>MKASLTFSLSGIYAPCSISRDIYLEYGDKKAECLYGTIRLPQYGPGCTPGKIVHCVLDDSLPFCSIVVPSKLFGFMPTQPTMDFCYFEPILDNVVPVLDSVTFLINEQLYSKLMDLPQEMQQIQFLHYKYNINSMETVVHSRDILTSGLCQILNCSPFPQGLVDFTETQLILVNDTEQKLSALKYANEDEEYALPKIGTNSALSIDLESLPCTISRDLLRPAPHINDDNSIYAFTDAETLLRLDVTSGSFITVSNMGCVRLVKLFVLLLPNGFKKRTIYAPPKIIASFPDCSVVTISKSNIGHTDIPIANQVFISRVGGWLQSQKCFQNIILTTLKKFFSESKRILCQNDLIPIAFDSSMADLNIAEENDESDDEDELGQYYKNDSLVWFFVTSAELDCFSKDNSHFIIDPNRTKLITTNITNRRPLPLSRSNLQRYYGFAETFYYDLHIFPYVRQLVNILETSFNCSQRGITLNASVLLHSTTNNVGKATMVRFASKYLGIHLLEIDCLSLTSNSRQLDSTSKIIGYIRAKCENVLPYASPAVIFLAHLDSILLDVNANQDPEAIKLQKSINFEMSKLLDDFTFKFPGTTFVGSVNNIDNVPSSFRSHMRFEILVPVPSEAQRLRIFQWYLSSHELNRDVQQKVPVSYMDNISFSSLSSYSAGLTPLDIKSIVETARMTATARFYQESKKCGWLPQSILITQEDLSKATSKARNEFSVSIGAPQIPNVTWDDIGGIDFVKGEILDTIDMPLKHPELFTSGMKKRSGILFYGPPGTGKTLMAKAIATNFSLNFFSVKGPELLNMYIGESEANVRRVFQKAREAKPCVIFFDQIDSVAPKRGNQGDSGGVMDRIVSQLLAELDGMSTDADGVFVIGATNRPDLLDEALLRPGRFDKLLYLGIPDTDTKQLNILEALTRKFVLDNDVKLIELAKLCPFNYTGADFYALCSDAMLNAMSRIARMVEKKVSQHNELTGENISTRRWFDKIATKEDTKVVVKMEDFLKAQEQLTPSVSRAELNHYEAVRANFEGA[3x];>TILKNGAIQLLKKVILRSTVCKMDFPKDNLFVVYISDGAQLPSQKGYASIVKCSLRQSKKSDSDNKSVGIPSKKIGVFIKCDSQIPENHIALSSHLWDAFFTHPMNGAKIKLEFLQMNQANIISGRNATVNIKYFGKDVPTKSGDQYSKLLGGSLLTNNLILPTEQIIIEIKKGESEQQLCNLNEISNESVQWKVTQMGKEEVKDIIERHLPKHYHVKETGEVSRTSKDEDDFITVNSIKKEMVNYLTSPIIATPAIILDGKQGIGKTRLLKELINEVEKDHHIFVKYADCETLHETSNLDKTQKLIMEWCSFCYWYGPSLIVLDNVEALFGKPQANDGDPSNNGQWDNASKLLNFFINQVTKIFNKDNKRIRVLFSGKQKTQINPLLFDKHFVSETWSLRAPDKHARAKLLEYFFSKNQIMKLNRDLQFSDLSLETEGFSPLDLEIFTEKIFYDLQLERDCDNVVTRELFSKSLSAFTPSALRGVKLTKETNIKWGDIGALANAKDVLLETLEWPTKYEPIFVNCPLRLRSGILLYGYPGCGKTLLASAVAQQCGLNFISVKGPEILNKFIGASEQNIRELFERAQSVKPCILFFDEFDSIAPKRGHDSTGVTDRVVNQLLTQMDGAEGLDGVYILAATSRPDLIDSALLRPGRLDKSVICNIPTESERLDILQAIVNSKDKDTGQKKFALEKNADLKLIAEKTAGFSGADLQGLCYNAYLKSVHRWLSAADQSEVVPGNDNIEYFSINEHGRREENRLRLKTLLQQDVVHETKTSTSAASELTAVVTINDLLEACQETKPSISTSELVKLRGIYDRFQKDR[3x]

The double-ring AAA+ ATPase Pex1/Pex6 is required for peroxisomal receptor recycling and is essential for peroxisome formation. Pex1 and Pex6 are both composed of two N-terminal domains (N1 and N2) followed by two AAA cassettes, known as the D1 and D2 domains. Pex1/Pex6 is the only known double-ring heterohexamer of the type II AAA+ family, with both subunits capped by a unique pair of N-terminal domains. We used a Pex6 Walker B mutant (E832Q) and “trapped” the heterohexamer processing an endogenous substrate along the central channel formed by the active D2 ring.

The second cryo-EM structure of substrate-bound Pex1/Pex6_WB shows a dynamic state where both the D1 and D2 rings of Pex1/Pex6 have an asymmetric configuration. One of the Pex6(D1)/Pex1(D1) dimers thereby swings out. This results in an open central D1 channel with a diameter of 20 Å, approximately 5 Å larger than the symmetric D1 ring in the “single-seam” state. Interestingly, the outward Pex6(D1)/Pex1(D1) dimer is stacked on top of a compact characteristic pair of dislocated seam domains of the D2 ring Pex6(D2)(E)/Pex1(D2)(F). We therefore term this conformation as the “twin-seam” state of the complex. In the “twin-seam” state, only four alternating Pex6(D2) and Pex1(D2) domains (Pex6(A), Pex1(B), Pex6(C), Pex1(D)) form the substrate-interacting spiral staircase of pore loops 1. The “twin-seam” dimer Pex6(E)/Pex1(F) is dislocated from the central channel. The lowermost D2 domain of the staircase is thus bound to ADP and the “twin-seam” dimer is released from the staircase. Intriguingly, our analysis suggests that the nucleotide binding pocket (E) between the two “seam” domains remains bound to ATP. Intriguingly, the pore loops 1 of the “twin-seam” in the D2 ring are close together and almost at identical heights, which, at least to our knowledge, has not been observed for canonical ATPases bound to substrate.> SMYMSNPTVRIAFVGKYLQDAGDTYFSVLQCFEHCQIALQVRLDILYVDSEELEGPNADEARKALLGCDGIFVPGGFGNRGVDGKCAAAQV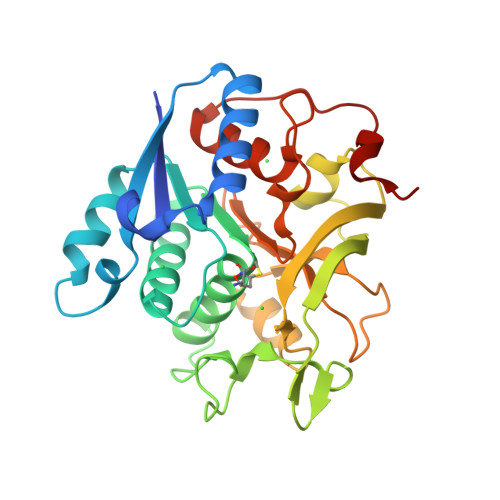ARMNNIPYFGVCLGMQVAVIELSRNVVGWSDANSEEFNKESTHQVVRIMDCDRNKMGANMHLGACDVYIVEKSSIMAKIYSKSNIVVERHRHRYEVNTAYFEDLRKAGLCISAVTDPTFSSRCRVEAVENPSLRFFLAVQFHPEFISTPMDPAPTYLSFMAAAAKKDYVWPQKCSQRRLKQA> MSYYHHHHHHLESTSLYKKAGMNTYGWDIVYGCSKRVVNKHLKEYITKNNIQFLYSNIDKKQEIKMVFDNWEIINGGSSNFLRIKTPIKEGYFKVRNTTVDLSGIN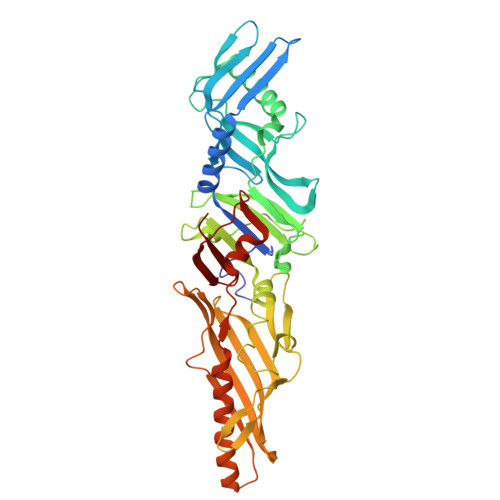PVLEIKLDFFNDISNPNIKELKFNFGSESNDDIKIIVSDLNGNLQEEDEFYFNKLLINAFIQNEKQISYIFASLNVTSDIEWMNPKQFKFVYYSPTDNSDGYLFILSVVTNRDISKLSANVDGNILGNNSEVGLLISEKLFLQNMVLSRLSSNMGSNINKNNFEVISTSDTTGRIVNNSTLNWYGLKVAALYYYPKINNFSMQLFEGNKLKISLRGLVRLTGLEAVYSDFEIQSINKFVYNSTNKKAYFEVDKNPTSSYKYHLFPGDLISLAVLSSVTHWSIKSIEGALGFELINNFVDLINNTIKWNNLKISQVTNVTLNVGFCIQGNAN In bacteria, cyclic dinucleotide (CDN)-based anti-phage signalling systems (CBASS) have been discovered. These systems are composed of cGAS-like enzymes and various effector proteins that kill bacteria on phage infection, thereby stopping phage spread. Using a genetic screen, we found that the phage protein Vs.4 antagonized cGAS signalling by binding tightly to cGAMP (dissociation constant of approximately 30 nM) and sequestering it. Vs.4 binds to cGAMP with a high affinity, thus sequestering cGAMP from its effector CapV, thereby enabling T4 phage to infect bacteria that do not produce enough cGAMP.

To further investigate this interaction, we determined the crystal structure of Vs.4 bound to cGAMP at a resolution of 2.0 Å. This structure revealed that Vs.4 formed a hexameric complex that bound to three cGAMP molecules. Analytical ultracentrifugation confirmed that Vs.4 formed a hexamer in solution. Within the hexamer, each cGAMP binding site is composed of two Vs.4 monomers, which make extensive π–π interactions between the purine bases of cGAMP and Y8/F82 of Vs.4. Extensive hydrogen bonds and salt bridges were observed between cGAMP and Y8, H11, K23 and R79 of Vs.4. Isothermal calorimetry (ITC) experiments showed that purified Vs.4 protein bound to cGAMP with a Kd of approximately 30 nM. To validate the experimental structure and to test the hypothesis that Vs.4 could bind cGAMP and sequester it from the effector protein CapV, we used an in vitro CapV activity assay, which showed that recombinant Vs.4 inhibited cGAMP-mediated activation of CapV. Importantly, we found that Vs.4 mutants harbouring mutations to either the cGAMP binding interface (Y8 and F82) or the hexamerization interfaces (L29, A66, A73 and A77) failed to inhibit CapV. Of the Vs.4 mutations identified from our forward genetic screen, A77I (which sterically clashes with the hexamerization interface), T12I (which removes a stabilizing helix cap) and S74N (which interferes with interactions with cGAMP) mutations were found to disrupt the ability of Vs.4 to inhibit CapV. We also found that mutations to the hexamerization interfaces (L29, A66, A73 and A77) abrogated cGAMP binding.

>[6x]SMIEDIKGYKPHTEEKIGKVNAIKDAEVRLGLIFDALYDEFWEALDNCEDCEFAKNYAESLDQLTIAKTKLKEASMWACRAVFQPEEKY>[2x]MFIKPGRCPKPAVQEDFDAARYLGVWYDIQRLPNKFQKG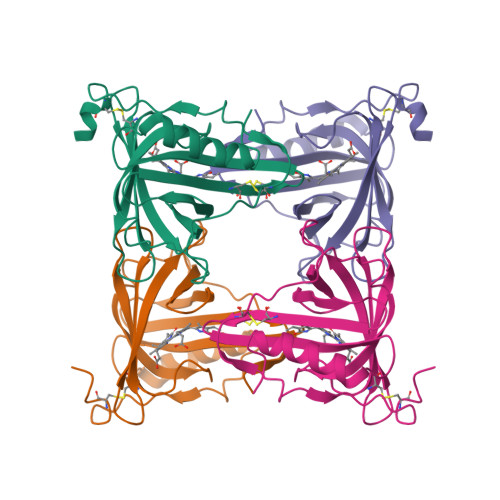ECATATYSLSPGVGFSVFNRERLANGTIKSVIGSAIAEDPCEPAKLQFFHENAAPVPYWVLSTDYDNYALVYSCINLGASHAAAASIVSRQPTLPEETIKKLQGTMSSFGVGVDTLLTTNQDAAYCSAMNQKLAAALEHHHHHH(3S)-4-({(1S)-2-[(8-aminooctyl)amino]-1-cyclobutyl-2-oxoethyl}amino)-3-hydroxy-4-oxobutanoic acid 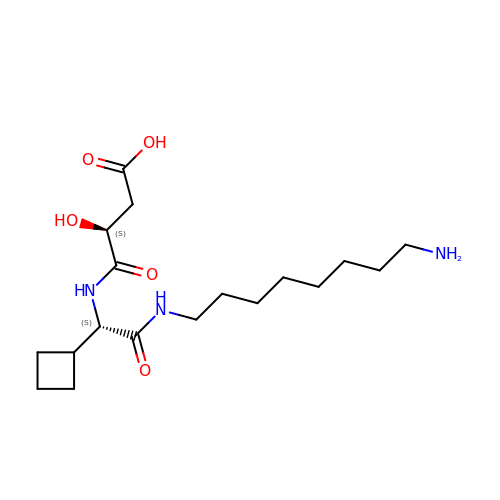| C18 H33 N3 O5 | DGPBSMLADVAZDL-HOCLYGCPSA-N>[4x]MGSSHHHHHHSQDPKPRVLVLTGAGISAESGIRTFRAADGLWEEHRVEDVGTPEGFDRDPELVQAFYNARRRQLQQPEIQPNAAHLALAKLQDALGDR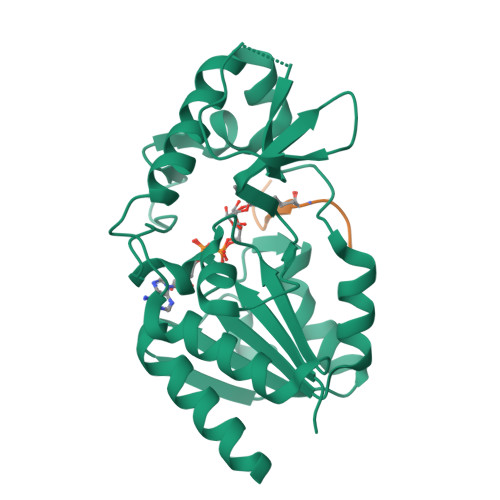FLLVTQNCDNLHERAGNTNVIHMHGELLKVRCSQSGQALDWTGDVTPEDKCHCCQFPAPLRPHVVWFGEMPLGMDEIYMALSMADIFIAIGTSGHVYPAAGFVHEAKLHGAHTVELNLEPSQVGNEFAEKYYGPASQVVPEFVEKLLKGLKAGSIA;>[4x]KGGAKRHRKIL>[2x]MSYKNATKPTETIMHANDAIQKTTASTRKPRLVVMVVGETARADHASFNGYQRATFPHMDK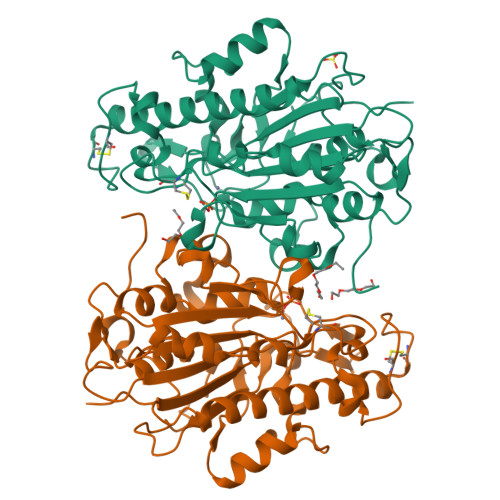LIGLGQVHNFGNVTSCGTSAAYSVPCMFSYLGAEKYDVDTADYHENVIDTLDRLGVAILWRDNNSDSKGVMNRLPAKQYQDYKNSPLQGGNNTICHTNPYDECRDVGMLVDLDDHVKAHANQDILIVLHQMGNHGPAYYKRYDDEFAQFLPVCTSSELAECERQTVINAYDNALLATDDFLKQTIDWLAAQTHADTAMLYLSDHGESLGEKGVYLHGMPKAFAPKEQLSIPALLWLGADTPFAVANSPTAGFSHDAITPTLLNLFDVSTQATADKTAFVNPLD Specialized protein transport systems—known as type VII secretion systems (T7SSs)—are central to the virulence of this pathogen, and are also crucial for nutrient and metabolite transport across the mycobacterial cell envelope. Mycobacterium tuberculosis encodes five homologous, but functionally distinct, T7SSs that are designated ESX-1 to ESX-5. These systems translocate a number of effector proteins across the unique and impermeable diderm cell envelope. Here we reconstituted the ESX-5 T7SS of M. tuberculosis H37Rv in M. smegmatis to obtain a structural view of the entire T7SS membrane complex from this human pathogen.

The intact machinery comprises EccB5, EccC5, EccD5, EccE5 and MycP5 with a 6:6:12:6:3 stoichiometry resulting in a 2.32-MDa complex that is anchored in the inner membrane through 165 transmembrane helices (TMHs). The membrane assembly is best described as a trimer of dimers, in which each dimer comprises a single copy of MycP5 and two protomers each of one copy of EccB5, EccC5, EccE5 and two copies of EccD5. We show how the 2.32-MDa ESX-5 assembly, which contains 165 transmembrane helices, is restructured and stabilized as a trimer of dimers by the MycP5 protease. A trimer of MycP5 caps a central periplasmic dome-like chamber that is formed by three EccB5 dimers, with the proteolytic sites of MycP5 facing towards the cavity. At the membrane level, six EccD5-dimer barrels (each of which contains 22 TMHs) together form a circular raft with an inner cavity. Within this raft, inner EccD5 monomers are situated closer to the centre, whereas outer EccD5 monomers face towards the periphery of the membrane complex. Instead, coupling between two neighbouring EccD5 barrels is achieved by the N-terminal loop and α-helix of EccB5 that run parallel to the cytoplasmic side of the inner membrane and engage in interactions with the TMHs of the neighbouring EccD5 barrel in a clockwise manner. We fully resolved the twelve EccC5 TMHs in the intact M. tuberculosis ESX-5 complex; these form three four-TMH bundles, each of which belongs to the EccC5 molecules of one dimer. These bundles are held together by hydrophobic interactions and effectively seal the central space of the membrane complex, which is enclosed by the EccB5 basket. The entrance to the putative EccC5 pore widens on the cytoplasmic side, where the EccC5 stalk domains expand radially. Together, our data suggest that the six EccD5 barrels provide a stable scaffold for assembly of a secretion pore that is confined by the EccB5 TMHs and gated through three EccC5 TMH bundles.

>MAEESRGQRGSGYGLGLSTRTQVTGYQFLARRTAMALTRWRVRMEIEPGRRQTLAVVASVSAALVICLGALLWSFISPSGQLNESPIIADRDSGALYVRVGDRLYPALNLASARLITGRPDNPHLVRSSQIATMPRGPLVGIPGAPSSFSPKSPPASSWLVCDTVATSSSIGSLQGVTVTVIDGTPDLTGHRQILSGSDAVVLRYGGDAWVIREGRRSRIEPTNRAVLLPLGLTPEQVSQARPMSRALFDALPVGPELLVPEVPNAGGPATFPGAPGPIGTVIVTPQISGPQQYSLVLGDGVQTLPPLVAQILQNAGSAGNTKPLTVEPSTLAKMPVVNRLDLSAYPDNPLEVVDIREHPSTCWWWERTAGENRARVRVVSGPTIPVAATEMNKVVSLVKADTSGRQADQVYFGPDHANFVAVTGNNPGAQTSESLWWVTDAGARFGVEDSKEARDALGLTLTPSLAPWVALRLLPQGPTLSRADALVEHDTLPMDMTPAELVVPK[6x];>[6x]MKRGFARPTPEKPPVIKPENIVLSTPLSIPPPEGKPWWLIVVGVVVVGLLGGMVAMVFASGSHVFGGIGSIFPLFMMVGIMMMMFRGMGGGQQQMSRPKLDAMRAQFMLMLDMLRETAQESADSMDANYRWFHPAPNTLAAAVGSPRMWERKPDGKDLNFGVVRVGVGMTRPEVTWGEPQNMPTDIELEPVTGKALQEFGRYQSVVYNLPKMVSLLVEPWYALVGEREQVLGLMRAIICQLAFSHGPDHVQMIVVSSDLDQWDWVKWLPHFGDSRRHDAAGNARMVYTSVREFAAEQAELFAGRGSFTPRHASSSAQTPTPHTVIIADVDDPQWEYVISAEGVDGVTFFDLTGSSMWTDIPERKLQFDKTGVIEALPRDRDTWMVIDDKAWFFALTDQVSIAEAEEFAQKLAQWRLAEAYEEIGQRVAHIGARDILSYYGIDDPGNIDFDSLWASRTDTMGRSRLRAPFGNRSDNGELLFLDMKSLDEGGDGPHGVMSGTTGSGKSTLVRTVIESLMLSHPPEELQFVLADLKGGSAVKPFAGVPHVSRIITDLEEDQALMERFLDALWGEIARRKAICDSAGVDDAKEYNSVRARMRARGQDMAPLPMLVVVIDEFYEWFRIMPTAVDVLDSIGRQGRAYWIHLMMASQTIESRAEKLMENMGYRLVLKARTAGAAQAAGVPNAVNLPAQAGLGYFRKSLEDIIRFQAEFLWRDYFQPGVSIDGEEAPALVHSIDYIRPQLFTNSFTPLEVSVGGPDIEPVVAQPNGEVLESDDIEGGEDEDEEGVRTPKVGTVIIDQLRKIKFEPYRLWQPPLTQPVAIDDLVNRFLGRPWHKEYGSACNLVFPIGIIDRPYKHDQPPWTVDTSGPGANVLILGAGGSGKTTALQTLICSAALTHTPQQVQFYCLAYSSTALTTVSRIPHVGEVAGPTDPYGVRRTVAELLALVRERKRSFLECGIASMEMFRRRKFGGEAGPVPDDGFGDVYLVIDNYRALAEENEVLIEQVNVIINQGPSFGVHVVVTADRESELRPPVRSGFGSRIELRLAAVEDAKLVRSRFAKDVPVKPGRGMVAVNYVRLDSDPQAGLHTLVARPALGSTPDNVFECDSVVAAVSRLTSAQAPPVRRLPARFGVEQVRELASRDTRQGVGAGGIAWAISELDLAPVYLNFAENSHLMVTGRRECGRTTTLATIMSEIGRLYAPGASSAPPPAPGRPSAQVWLVDPRRQLLTALGSDYVERFAYNLDGVVAMMGELAAALAGREPPPGLSAEELLSRSWWSGPEIFLIVDDIQQLPPGFDSPLHKAVPFVNRAADVGLHVIVTRTFGGWSSAGSDPMLRALHQANAPLLVMDADPDEGFIRGKMKGGPLPRGRGLLMAEDTGVFVQVAATEVRR;>[12x]MTAVADAPQADIEGVASPQAVVVGVMAGEGVQIGVLLDANAPVSVMTDPLLKVVNSRLRELGEAPLEATGRGRWALCLVDGAPLRATQSLTEQDVYDGDRLWIRFIADTERRSQVIEHISTAVASDLSKRFARIDPIVAVQVGASMVATGVVLATGVLGWWRWHHNTWLTTIYTAVIGVLVLAVAMLLLMRAKTDADRRVADIMLMSAIMPVTVAAAAAPPGPVGSPQAVLGFGVLTVAAALALRFTGRRLGIYTTIVIIGALTMLAALARMVAATSAVTLLSSLLLICVVAYHAAPALSRRLAGIRLPVFPSATSRWVFEARPDLPTTVVVSGGSAPVLEGPSSVRDVLLQAERARSFLSGLLTGLGVMVVVCMTSLCDPHTGQRWLPLILAGFTSGFLLLRGRSYVDRWQSITLAGTAVIIAAAVCVRYALELSSPLAVSIVAAILVLLPAAGMAAAAHVPHTIYSPLFRKFVEWIEYLCLMPIFPLALWLMNVYAAIRYR;>MQRFGTGSSRSWCGRAGTATIAAVLLASGALTGLPPAYAISPPTIDPGALPPDGPPGPLAPMKQNAYCTEVGVLPGTDFQLQPKYMEMLNLNEAWQFGRGDGVKVAVIDTGVTPHPRLPRLIPGGDYVMAGGDGLSDCDAHGTLVASMIAAVPANGAVPLPSVPRRPVTIPTTETPPPPQTVTLSPVPPQTVTVIPAPPPEEGVPPGAPVPGPEPPPAPGPQPPAVDRGGGTVTVPSYSGGRKIAPIDNPRNPHPSAPSPALGPPPDAFSGIAPGVEIISIRQSSQAFGLKDPYTGDEDPQTAQKIDNVETMARAIVHAANMGASVINISDVMCMSARNVIDQRALGAAVHYAAVDKDAVIVAAAGDGSKKDCKQNPIFDPLQPDDPRAWNAVTTVVTPSWFHDYVLTVGAVDANGQPLSKMSIAGPWVSISAPGTDVVGLSPRDDGLINAIDGPDNSLLVPAGTSFSAAIVSGVAALVRAKFPELSAYQIINRLIHTARPPARGVDNQVGYGVVDPVAALTWDVPKGPAEPPKQLSAPLVVPQPPAPRDMVPIWVAAGGLAGALLIGGAVFGTATLMRRSRKQQ[3x]>[4x]GSHMTDLAGPTITPNLQLVYVSNVERSTDFYRFIFKKEPVFVTPRYVAFPSSGDALFAIWSGGEEPVAEIPRFSEIGIMLPTGEDVDKLFNEWTKQKSHQIIVIKEPYTDVFGRTFLISDPDGHIIRVCPLD

Enterobacter agglomerans strain Eh1087 generates the phenazine antibiotic D-alanyl griseoluteic acid to compete with other microorganisms in its habitat. In order to protect itself against the toxic action of this compound, the bacterium produces the resistance protein EhpR together with enzymes required for phenazine biosynthesis. EhpR belongs to the glyoxalase I/bleomycin resistance protein family, whose members have a wide variety of functions extending from simple binding of toxic small molecules to their chemical conversion through enzymatic activity. The EhpR monomer consists of two βαββ'β fold units (' indicating antiparallel orientation with respect to the other strands) that are typical for members of the glyoxalase I/bleomycin resistance protein family.

EhpR behaved as a homodimer during size exclusion chromatography and crystallized in space group P212121 with two and one dimers per asymmetric unit in the apo and GA-cocrystallized form, respectively. The structure was solved from single-wavelength anomalous diffraction data collected at the K-edge of seleno-L-methionine labeled protein crystallized in the apo form. These crystals diffracted to 2.15 Å and the structure was refined to a crystallographic R-factor of 20.5% with Rfree = 25.9%. Also noteworthy in the EhpR dimer are the extended N-termini, which give rise to an "arm exchange" between the two monomers. While these arms are too flexible to be traced beyond G6 in the apo structure, all residues including those remaining from the N-terminal His6-tag after thrombin cleavage could be traced in the atomic resolution data set. While the apo and complex structure are otherwise highly similar (average rmsd < 0.6 Å over the complete monomer), F109* undergoes a significant conformational and positional change on ligand binding. It adopts a different rotamer and moves together with the loop from E103 to G110, which leads to the formation of an open conformation of the ligand binding site with respect to the apo structure. This movement is required to unblock the binding site and suggests that ligand binding follows a multi-step mechanism. In addition, the finding that the binding site is blocked by F109 in the apo structure indicates that the ligand needs to induce structural rearrangements.>MSVAYNPQTKQFHLRAGKASYVMQLFRSGYLAHVYWGKAVRDVRGARAFPRLDRAFSPNPDPSDRTFSLDTLLQEYPAYGNTDFRAPAYQVQLENGSTVTDLRYKTHRIYKGKPRLNGLPATYVEHEQEAETLEIVLGDALIGLEVTLQYTAYEKWNVITRSARFENKGGERLKLLRALSMSVDFPTADYDWIHLPGAWGRERWIERRPLVTGVQAAESRRGASSHQQNPFIALVAKNADEHQGEVYGFSFVYSGNFLAQIEVDQFGTARVSMGINPFDFTWLLQPGESFQTPEVVMVYSDQGLNGMSQTYHELYRTRLARGAFRDRERPILINNWEATYFDFNEEKIVNIARTEAELGIELVVLDDGWFGERDDDRRSLGDWIVNRRKLPNGLDGLAKQVNELGLQFGLWVEPEMVSPNSELYRKHPDWCLHVPNRPRSEGRNQLVLDYSREDVCDYIIETISNVLASAPITYVKWDMNRHMTEIGSSALPPERQRETAHRYMLGLYRVMDEITSRLPHILFESCSGGGGRFDPGMLYYMPQTWTSDNTDAVSRLKIQYGTSLVYPISAMGAHVSAVPNHQVGRVASLKTRGHVAMSGNFGYELDITKLTETEKQMMKQQVAFYKDVRRLVQFGTFYRLLSPFEGNEAAWMFVSADRSEALVAYFRVLAEANAPLSYLRLKGLDSNQDYEIEGLGVYGGDELVYAGVALPYRSS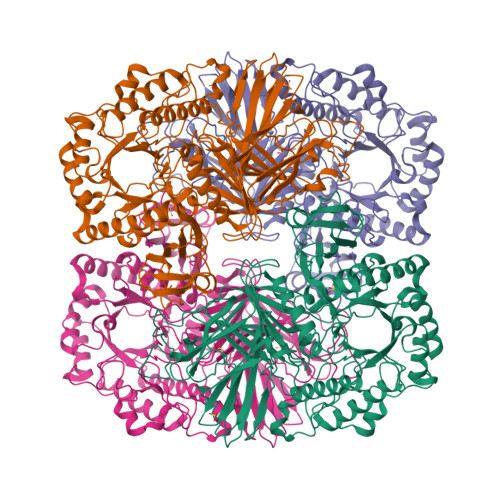DFISMMWRLKAVQQ[4x]> MTGDHIKVIYFNGRGRAESIRMTLVAAGVNYEDERISFQDWPKIKPTIPGGRLPAVKITDNHGHVKWMVESLAIARYMAKKHHMMGGTEEEYYNVEKLIGQAEDLEHEYYKTLMKPEEEKQKIIKEI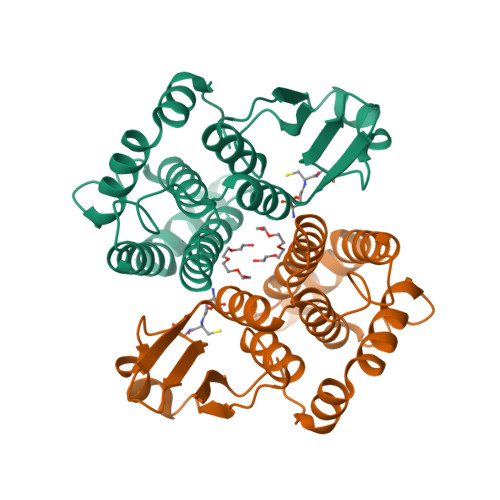LNGKVPVLLDIICESLKASTGKLAVGDKVTLADLVLIAVIDHVTDLDKEFLTGKYPEIHKHRENLLASSPRLAKYLSDRAATPF Here we present aficamten, a selective small-molecule inhibitor of cardiac myosin that diminishes ATPase activity by strongly slowing phosphate release, stabilizing a weak actin-binding state. Binding to an allosteric site on the myosin catalytic domain distinct from mavacamten, aficamten prevents the conformational changes necessary to enter the strongly actin-bound force-generating state. In doing so, aficamten reduces the number of functional myosin heads driving sarcomere shortening. The crystal structure of aficamten bound to cardiac myosin in the pre-powerstroke state provides a basis for understanding its selectivity over smooth and fast skeletal muscle.

To better define the mechanism of action of aficamten and to explain its specificity for β-MHC, we co-crystallized β-MHC with aficamten and Mg.ADP.Vanadate. The structure solved at 2.33 Å resolution revealed that two β-MHC motor domain molecules were trapped in the pre-powerstroke (PPS) state in the asymmetric unit. The electron density map unambiguously identified the position of aficamten and the nucleotide in both molecules. As suspected from competition assays, aficamten targets the same pocket as blebbistatin, located between the U50 (upper 50 kDa) and the L50 (lower 50 kDa) subdomains in close vicinity to the inorganic phosphate (Pi)-release backdoor. Little conformational change occurs upon aficamten binding, the primary difference being a new position of the Leu267 side chain. A more detailed analysis of the pocket shows that most of the interactions are hydrophobic in nature with only two electrostatic interactions. The first electrostatic bond involves the carboxyl group of the L267 main chain that forms a hydrogen bond with the N–H moiety from the amide bond between the pyrazole and indane of aficamten. The second electrostatic interaction involves a hydrogen bond network between a water molecule with the nitrogen from the imidazole of H651 and a side chain NH2 of N654 of β-MHC and nitrogen 4 of the oxadiazole from aficamten. Despite binding to the same site as the nonselective inhibitor blebbistatin, notably aficamten is selective for cardiac β-MHC relative to smooth and fast skeletal muscle myosin. Specificity is likely achieved through the above-mentioned second electrostatic interaction involving a water-mediated hydrogen bond to residues CarH651 and CarN654 of β-MHC and nitrogen 4 of the oxadiazole from aficamten. Inhibition of ATPase activity by the compounds results from prevention of rearrangements of the myosin internal cleft, which are required to change the actin interface and thus the release of the hydrolysis products.

>[2x]MVDAEMAAFGEAAPYLRKSEKERLEAQTRPFDLKKDVFVPDDKEEFVKATILSREGGKVTAETEHGKTVTVKEDQVLQQNPPKFDKIEDMAMLTFLHEPAVLYNLKERYASWMIYTYSGLFCVTINPYKWLPVYNAEVVAAYRGKKRSEAPPHIFSISDNAYQYMLTDRENQSILITGESGAGKTVNTKRVIQYFAVIAAIGDRSKKEQATGKGTLEDQIIQANPALEAFGNAKTVRNDNSSRFGKFIRIHFGATGKLASADIETYLLEKSRVIFQLKAERDYHIFYQILSNKKPELLDMLLITNNPYDYAFISQGETTVASIDDAEELMATDNAFDVLGFTTEEKNSMYKLTGAIMHFGNMKFKLKQREEQAEPDGTEEADKSAYLMGLNSADLLKGLCHPRVKVGNEYVTKGQNVQQVVYAKGALAKAVYERMFNWMVTRINATLETKQPRQYFIGVLDIAGFEIFDFNSFEQLCINFTNEKLQQFFNHHMFVLEQEEYKKEGIEWEFIDFGMDLQACIDLIEKPMGIMSILEEECMFPKATDMTFKAKLFDNHLGKSSNFQKPRNIKGKPEAHFSLIHYAGTVDYNIIGWLQKNKDPLNETVVDLYKKSSLKMLSSLFANYAGFDTPIEKGKGKAKKGSSFQTVSALHRENLNKLMTNLRSTHPHFVRCIIPNETKSPGVIDNPLVMHQLRCNGVLEGIRICRKGFPNRILYGDFRQRYRILNPAAIPEGQFIDSRKGAEKLLGSLDIDHNQYKFGHTKVFFKAGLLGLLEEMRDERLS>[6x]MKIGSVIESSPHSILVKIDTLKIFEKAKSALQIGKYLKIQEGNHNFVLCVIQNIKISTDKDEDIFILTVQPVGIFKGEEFFQGNSMLPSPTEPVFLVEDDILNKIFSNEKTKIFHLGNLAQNEEVSFTLDGDKFFSKHVAVVGSTGSGKSCAVAKILQNVVGINDARNI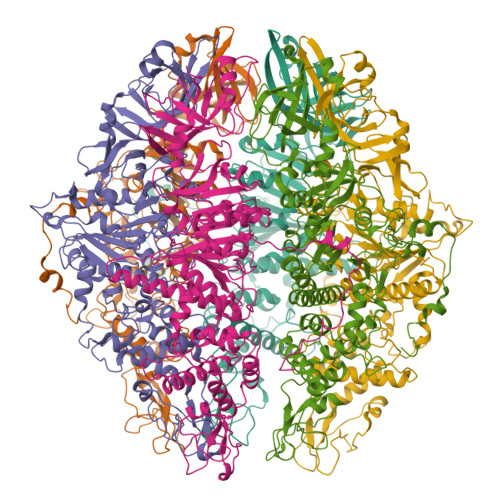NKSDKKNSHIIIFDIHSEYKSAFEIDKNEDFNLNYLDVEKLKLPYWLMNSEELETLFIESNEQNSHNQVSQFKRAVVLNKEKYNPEFKKITYDSPVYFNINEVFNYIYNLNEEVINKIEGEPSLPKLSNGELVENRQIYFNEKLEFTSSNTSKATKASNGPFNGEFNRFLSRFETKLTDKRLEFLLLNQDVEENSKYRTEHFEDILKQFMGYLDRSNVSIIDLSGIPFEVLSITISLISRLIFDFAFHYSKLQHQKDELNDIPFMIVCEEAHNYIPRTGGIEFKAAKKSIERIAKEGRKYGLSLMVVSQRPSEVSDTILSQCNNFINLRLTNINDQNYIKNLLPDNSRSISEILPTLGAGECLVVGDSTPIPSIVKLELPNPEPRSQSIKFHKKWSESWRTPSFEEVIMRWRKENG>[2x]MLYIDEFKEAIDKGYILGDTVAIVRKNGKIFDYVLPHEKVRD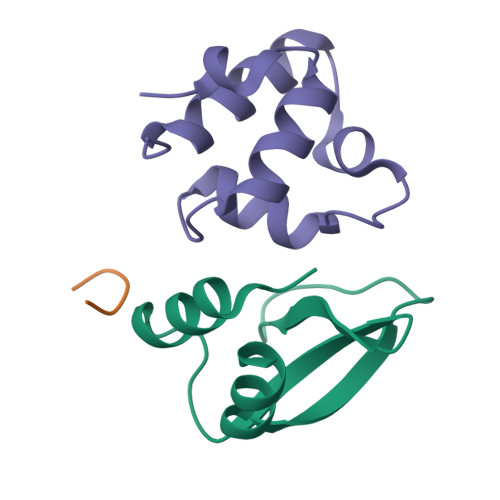DEVVTVERVEEVMVELDKLEHHHHHH;> GSHMLKDFGKKIKSLRLEKGLTKEAVCLDESQLSTRQLTRIESGQSTPTLNKAVYIAGRLGVTLGYLTD> MGKVIRSLNRFGKKVGNALTSNTAKKIYSTIGKAAERFAESEIGSAAIDGLVQGSVHSIITGESYGESVKQAVLLNVLGSGEEIPDPLSPGERGIQAKLKELEDEQRNELVRLKYNDKIKEKFGKELEEVYNFMNGEANAEIEDEKQFDILNKAVTSYNKILTEEDLQMRRLATALQKEIGERTHAETVMVKEYRDKIDALKNAIEVERDGMQEEAIQEIAGMTADVLEAASEEVPLIGAGMATAVATGRAIEGAYKLKKVINALSGIDLTHLRTPKIEPSVVSTILEYRAKEIPDNALAVSVLSKNRAIQENHKELMHIKNEILPRFKKAMDEEKEICGIEDKVIHPKVMMKFKIPRAQQPQIHVYSAPWDSDDVFFFHCISHHHANESFFLGFDLSIDLVHYEDLTAHWHALGAAQTAAGRTLTEAYREFLNLAISNAFGT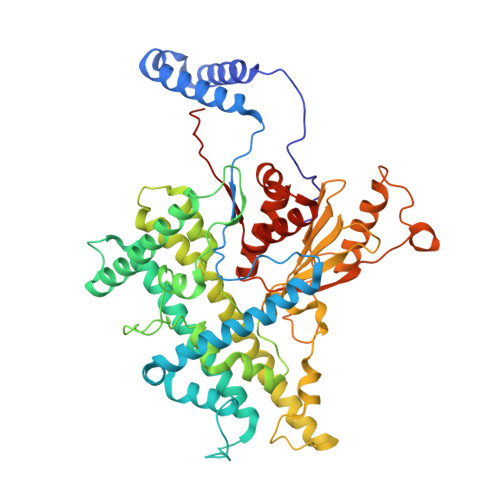QMHTRRLVRSKTVHPIYLGSLHYDISFSDLRGNAQRIVYDDELQMHILRGPIHFQRRAILGALKFGCKVLGDRLDVPLFLRNA>RPKLYVMDNGRMRMDKNWMIAMHNPATIHNPNAQTEFVEFPIYTVLIDHPEGKILFDTSCNPNSMGPQGRWAESTQQMFPWTATEECYLHNRLEQLKVRPEDIRYVVASHLHLNHAGCLEMFTNATIIVHEDEFNGALQCYARNQKEGAYIWADIDAWIKNNLQWRTVKRHEDNILLAEGVKVLNFGSGHAWGMLGLHVELPETGGIILASDAIYTAESYGPPIKPPGIIYDSLGYMNTVERIRRIAQETKSQVWFGHDAEQFKKFRKSTEGYYE[2x]

MLLs degrade N-acyl-L-homoserine lactones (AHLs), molecules that are used in a microbial communication system called quorum sensing (QS) to coordinate a variety of behaviors, including virulence and biofilm formation. We provide the structural and biochemical analysis of the lactonase GcL (WP_017434252.1), isolated from the thermophilic bacteria Parageobacillus caldoxylosilyticus. GcL is a thermostable, highly proficient lactonase with broad substrate specificity (kcat/KM values range between 104 to 106 M–1 s–1) for substrates such as N-butyryl (C4) L-homoserine lactone (HSL) and N-decanoyl (C10)-HSL. The binuclear center, common to all MLLs, is coordinated by five histidine residues and two aspartic acid residues.

Asp122 is also conserved and is involved in coordinating the metal cation. To investigate the importance of these residues, we therefore substituted Tyr223 with phenylalanine and Asp122 with asparagine in GcL, eliminating their role in acid catalysis, and kinetically characterized the resulting GcL variants. The alterations in GcL activity may still suggest that this residue is important, but the interpretation of this effect is complicated by the clear role of this residue in metal coordination. This could be seen through crystallization, where multiple conformations were captured: one where both metals are present at high occupancy, exhibiting an active site configuration very similar to that of the wild-type enzyme; and a second form where the active site shows no bound β-metal (or bound with very low occupancy). In the case of the Asp122Asn variant, the Asp mechanism is no longer accessible due to the mutation of Asp122, leaving only the terminal hydroxide or concerted mechanisms as potential options. Curiously, in this variant, the activation free energy for the terminal hydroxide mechanism increases substantially, leaving the concerted mechanism as the only energetically plausible pathway with calculated activation free energies within 3 kcal mol–1 of the experimental data. Visual examination of our EVB trajectories indicates that during our simulations, the substituted N122 side chain interacts with and stabilizes the terminal hydroxide ion at the Michaelis complex, contributing to higher calculated activation free energies through reactant state stabilization.> AIGEFMVSLPRMVYPQPKVLTPCRKDVLVVTPWLAPIVWEGTFNIDILNEQFRLQNTTIGLTVFAIKKYVAFLKLFLETAEKHFMVGHRVHYYVFTDQPAAVPRVTLGTGRQLSVLEVGAYKRWQDVSMRRMEMISDFCERRFLSEVDYLVCVDVDREFRDHVGVEILTP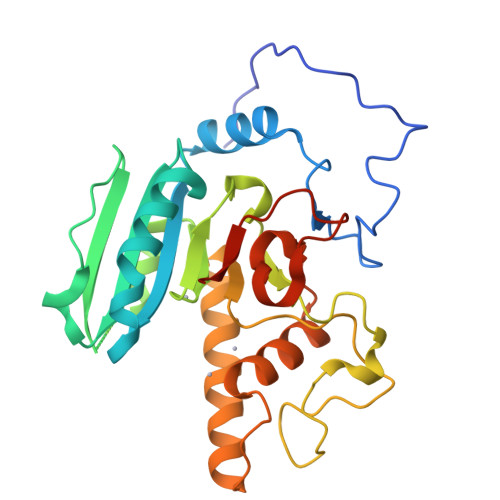LFGTLHPSFYGSSREAFTYERRPQSQAYIPKDEGDFYYMGAFFGGSVQEVQRLTRACHQAMMVDQANGIEAVWHDESHLNKYLLRHKPTKVLSPEYLWDQQLLGWPAVLRKLRFTAVPKNHQAVRNP>MSSEEKRLIKLPRTHKDGHLFEVSEAAIDWIEQYQHFKGVTKSIVELMNLISLRGLRSRDG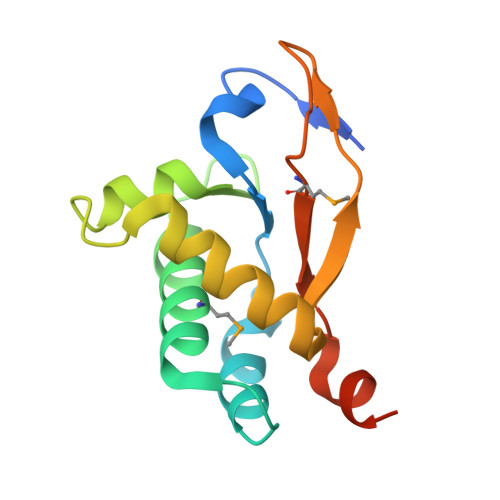LVSTTELIDATDGQLTRAAIQQRLRAAVAVGLFKQIPVRFEEGLAGKTMLHRFINPNQLISVLHHHHHH[2x]>GSTVPYTITVNGTSQNILSNLTFNKNQNISYKDLEGKVKSVLESNRGITDVDLRLSKQAKYTVNFKNGTKKVIDLKSGIYTA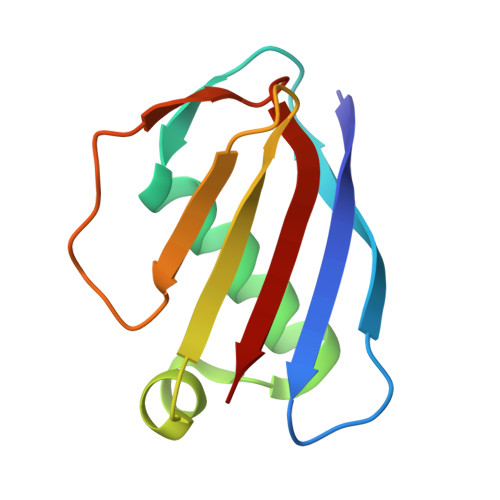NLINSSDIKSININID[2x]>MRDLKDIPEWRRIPKGENSVAACFGPRGGFKNFGDAEFVEKGVDASGYAQIASLAPNVAALLFGGNVAVRELADSYEITYNYKMTVPKSDPN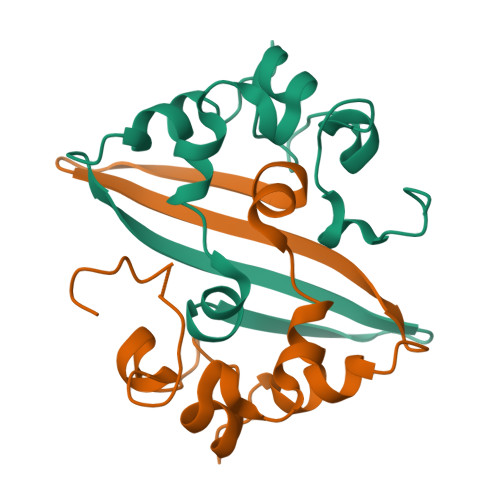VELLVSQVDAFKLEHHHHHHHH[8x]succinimide | C4 H3 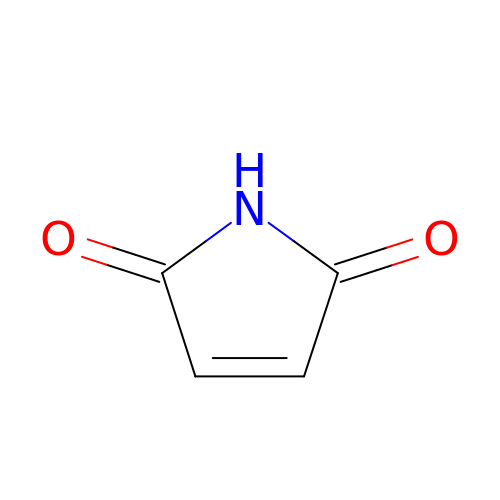N O2 | PEEHTFAAVSWFBL-UHFFFAOYSA-N EPDR1 is a member of the ependymin-related (EPDR) family of proteins. The crystal structure confirms that EPDR1 adopts the highly curved β-sheet fold that had been previously observed only in bacterial proteins. Two EPDR1 chains associate into a tight homodimer through extensive hydrophilic contacts between the convex surfaces of shelf-II. At acidic pH, EPDR1 can bind to liposomes that contain the anionic lipid bis-monoacylglycero-phosphate (BMP) or the ganglioside GM1, consistent with a role in the degradation or transport of lipids and/or lipoproteins within the lysosome.

We solved the deglycosylated form by Se-Met SAD phasing and used this structure to solve the glycosylated form by molecular replacement. Deglycosylated EPDR1 crystallized in a different packing arrangement with two independent homodimers per asymmetric unit. All three of the crystallographically independent EPDR1 homodimers (one dimer from crystals of the glycosylated protein, and two dimers from crystals of the deglycosylated protein) are similar to each other with Cα RSMDs less than 0.6 Å, indicating little variability within the chains and across the homodimer interface. The main difference between the structures from the two crystal forms is that no ligands were observed within the pockets in any of the deglycosylated structures, and we refer to the deglycosylated structures as apo-EPDR1. In addition to the empty ligand pockets, the loops at the mouth of the groove of apo-EPDR1 had weaker electron density. This is reflected in the higher atomic displacement parameters for loops L6 and L7, while L9, L4 and the C-terminal half of L12 (the latter two are linked by a disulfide bond between residues C88 and C222) could not be traced at all. We suggest that the ridge that lines the opening to the ligand groove is dynamic and flexible in apo-EPDR1 and becomes more ordered upon the binding of a ligand.

>[4x]SAPRPCQAPQQWEGRQVMYQQSSGRNSRALLSYDGLNQRVRVLDERKALIPCKRLFEYILLYKDGVMFQIDQATKQCSKMTLTQPWDPLDIPQNSTFEDQYSIGGPQEQITVQEWSDRKSARSYETWIGIYTVKDCYPVQETFTINYSVILSTRFFDIQLGIKDPSVFTPPSTCQMAQLEKMSEDCSWHHHHHH> MDLPYYHGCLTKRECEALLLKGGV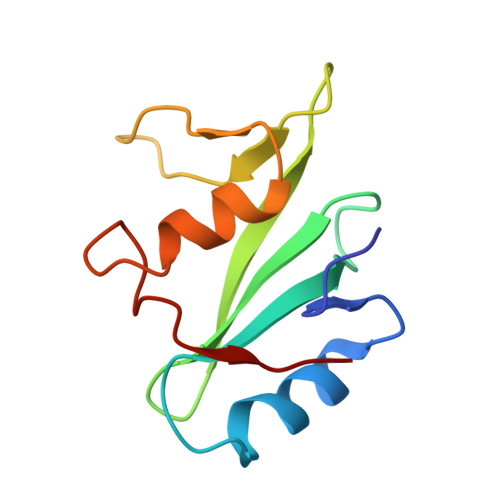DGNFLIRDSESVPGALCLCVSFKKLVYSYRIFREKHGYYRIETDAHTPRTIFPNLQELVSKYGKPGQGLVVHLSNPIMR>TALAEMPKRKFTIDDFDIGRPLGKGKFGNVYLAREKQNKFIMALKVLFKSQLEKEGVEHQLRREIEIQSHLRHPNILRMYNYFHDRKRIYLMLEFAPRGELYKELQKHGRFDEQRSATFMEELADALHYCHERKVIHRDIKPENLLMGYKGELKIADFGWSVHAPSLRRRTMCGTLDYLPPEMIEGKTHDEKVDLWCAGVLCYEFLVGMPPFDSPSHTETHRRIVNVDLKFPPFLSDGSKDLISKLLRYHPPQRLPLKGVMEHPWVKANSRRVLPPVYQ[2x];>[2x]IPIPAWASGNLLTQAIRQQYYKPIDVDRMYGTIDSPKLEELFNKSKPRYFKR

The Aurora family is a well conserved and well characterized group of serine-threonine kinases involved in the normal progression of mitosis. Mammalian cells possess three Aurora kinase isoforms (Aurora A, B and C) that exhibit different subcellular localizations and have distinct functional roles. The most conserved C-terminal region of INCENP (the so-called IN-box) is sufficient to bind and stimulate the catalytic activity of Aurora B. The CPC complex is involved in numerous mitotic functions, and the timing and mechanisms of each of these events are carefully regulated by its localization within mitosis. As expected, deregulation of Aurora kinases has drastic intra­cellular consequences, rendering these kinases attractive drug targets for small-molecule inhibitor development, targeting the active-site binding pocket which binds the ATP substrate.

We sought to investigate this further, and grew crystals of Aurora B–INCENP in the presence of a nonhydrolyzable ATP analogue (AMP-PNP). We also report the structure of the same complex bound to a nonhydrolyzable nucleotide that induces the formation of a crystal contact mediated by the substrate-recognition region of Aurora B and a neighbouring INCENP molecule. The C-terminus of a neighbouring INCENP molecule occupies the Aurora B substrate-binding region of an adjacient symmetry mate. An unexpected crystal-packing contact in the Aurora B–INCENP structure coordinated by an ATP analogue is also reported, in which the INCENP C-­terminus occupies the substrate-binding region, resembling the protein kinase A inhibitory mechanism. During the structure refinement, we were intrigued by the precise docking of the INCENP C-terminus onto the Aurora B substrate-recognition region. Although unexpected, the crystal contact favoured by the presence of a nucleotide within the Aurora B ATP-binding cleft may resemble the inhibitory mechanism observed for protein kinase A (PKA), in which an inhibitor protein (PKI) was originally co-discovered. Our structural data predict that phosphorylation of the TSS motif would disfavour its proximity to the pThr248Aurora B residue on the activation loop.>MGKAVIAIHGGAGAISRAQMSLQQELRYIEALSAIVETGQKMLEAGESALDVVTEAVRLLEECPLFNAGIGAVFTRDETHELDACVMDGNTLKAGAVAGVSHLRNPVLAARLVMEQSPHVMMIGEGAENFAFARGMERVSPEIFSTSLRYEQLLAARKEGATVLDHSGAPLDEKQKMG[2x];>[2x]TVGAVALDLDGNLAAATSTGGMTNKLPSTVGSSPLVGAGCYANNASVAVSCTGTGEVFIRALAAYDIAALMDYGGLSLAEACERVVMEKLPALGGSGGLIAIDHEGNVALPFNTEGMYRAWGYAGDTPTTGIYREKGDTVATQ

l-Asparaginases hydrolyze l-asparagine to l-aspartic acid and ammonia. The prototypic class 2 enzyme is EcAIII from E. coli. EcAIII belongs to the Ntn-hydrolases, which are expressed as immature polypeptides that dimerize and then autocatalytically cleave themselves into α (∼20 kDa) and β (∼15 kDa) subunits to form the mature (αβ)2 heterotetramer (a dimer of two αβ heterodimers). The same Thr179 acts as the nucleophile in the autoproteolytic maturation and in l-asparagine hydrolysis.

Mutant RDM1-37 has a serine instead of Asp at position 210. Its Oγ atom is hydrogen-bonded via two water molecules to the side chain of Ser211, which was not replaced in this variant. Of particular interest is the case of RDM1-43, which has the same D210S substitution as mutant RDM1-37, and yet in contrast to the latter variant lost its ability to autocleave. In both RDM1-43 and RDM1-37 Ser at position 211 was preserved. Mutants RDM1-37 and RDM1-43 differ in the type of substitutions at positions 206 and 207 (206→S/V and 207→T/G, respectively). It is possible that these two differences changed the mobility (conformational disorder) of the linker and significantly lowered the probability of proper conformation and orientation at the scissile bond. Asp210 and Ser211 could be substituted individually (variant RDM1-37, D210S mutation only) or simultaneously (variants RDM1-3, RDM1-8, RDM1-12, RDM1-18, RDM1-24, RDM1-29 and RDM1-38) without any loss of autocatalytic activity.4-[4-[(4,4-dimethylpiperidin-1-yl)methyl]phenyl]-9-[6-(propan-2-ylamino)pyrimidin-4-yl]-1,4,9-triazaspiro[5.5]undecan-2-one 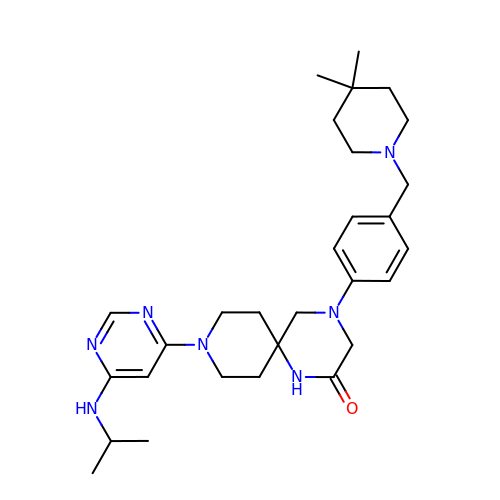| C29 H43 N7 O | HJOBOVGEKZTYKP-UHFFFAOYSA-N>AQYEDGKQYTTLEKPVAGAPQVLEFFSFFCPLCYQFEEVLHISDNVKKKLPEGVKMTKYHVNFMGGDLGKDLTQAWAVAMALGVEDKVTVPLFEGVQKTQTIRSASDIRDVFINAGIKGEEYDAAWNSFVVKSLVAQQEKAAADVQLRGVPAMFVNGKYQLNPQGMDTSNMDVFVQQY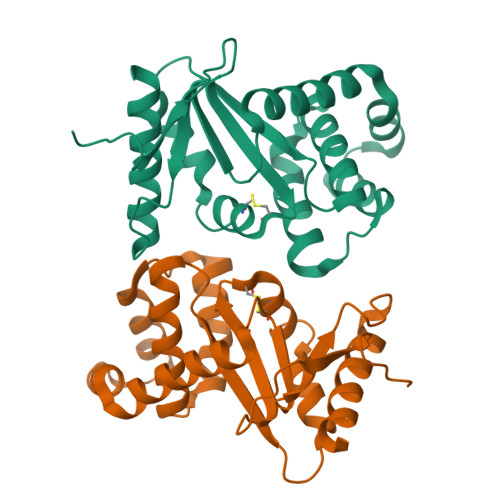ADTVKYLSEKK[2x]>[8x]MHHHHHHGSNKKSLSVIFVKPPFQLKKKFQKDPFYEIEMRKQLQMQQDGI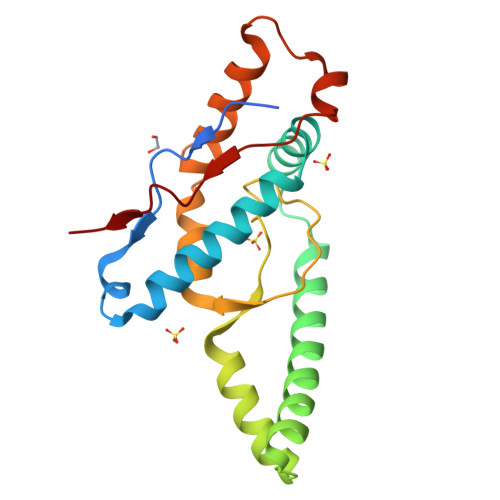NNMTIFEWLKNRENFKKYGRNPKSKKIQEDFRDRYRNAKIDEYLLLYEDMDIKAIEAMVDSELEGLAALANPAQIAGGYVDVVTQMGNKRINSSIGSQWGSIEKGRSLNIENELLKLITDPPPITEEEQKKIKMNVNLVENLEIVK> LDMSLNIHI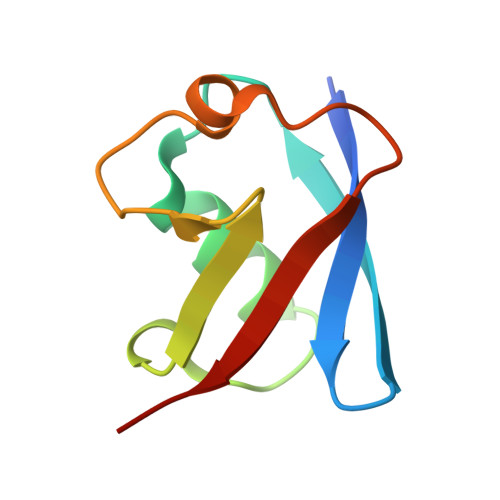KSGQDKWEVNVAPESTVLQFKEAINKANGIPVANQRLIYSGKILKDDQTVESYHIQDGHSVHLVKSQP>HHMQPQPSLKGHWTTKVIEKIGTFHDATSLYERVKKTCKYKYYYNDQVPNHVAVMRMTTSGINCTDACQLFSKVLEEMGYEVKIEHVRVKCNDGKWYGHYLLRVGGFELKDGTIWDYVSATKTGRPLGVPCCTAGFQHLGWGIVGPV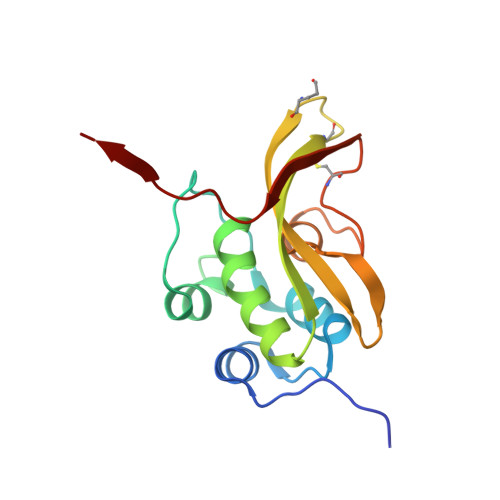YDK[4x]>GAMGSGIQRPTSTSSLVAAAMAEEEEVEEGRSSSSAILDLPEPLLLHILSFLTDVRSRHRAALACGRMRAAERATRSELSLRGDPRSPGFLFLSHAFRFPALEHLDLSLVSPWGHPLLSSVPPCGGGGGGAPSASSSSGMNVYHPEAISEQNAFIAARLAGCFPAVTSLAVYCRDPTTLANLTPHWQASLRRVKLVRWHQRPPTLPDGADLEPLLETCAALRELDLSEFYCWTEDVVRALTTHPSATAALTHLDLGLAAATDGFKSSELGPIAASCPNLRKLVAPCLFNPRFSDCVGDDALLSLATSCPRLTVLRLSEPFEAAANIQREEAAITVAGLVAFFAALPALEDFTMDLQHNVLEAAPAMEALARRCPRIKFLTLGSFQGLCKASWLHLDGVAVCGGLESLYMKNCQDLTDASLAAIGRGCRRLAKFGIHGCDLVTSAGIRRLAFTLRPTLKEVTVLHCRLLHTAECLTALSPIRDRIESLEINCVWNTTEQPCSVANGTTTECDPEDDELGEVYESAAKKCRYMEFDDLGSWEMLRSLSLWFSAGQLLSPLISAGLDSCPVLEEISIKVEGDCRTCPRPAPRTIFGL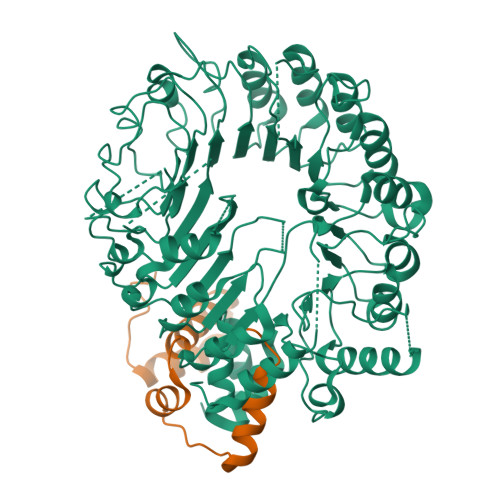SDLAGFPVLAKMKLDLSEAVGYALTAPTGQMDLSLWERFYLHGIESLQTLYELDYWPPQDKDVHHRSLTLPAVGLIQRCVGLRKLFIHGTTHEHFMTFFLSIPNLRDMQLREDYYPAPENDLMFTEMRAESWLRFEVQLNSRQIDD[2x];>MDYKDDDDKMSAKKIVLKSSDGESFEVEEAVALESQTIAHMVEDDCVDNGVPLPNVTSKILAKVIEYCKRHVEAAASKAEAVEGAATSDDDLKAWDADFMKIDQATLFELILAANYLNIKNLLDLTCQTVADMIKGKTPEEIRTTFNIKNDFTPEEEEEVRRENQWAFE[2x]N,N-dimethyl-3-(6-methyl-7-oxo-6,7-dihydro-1H-pyrrolo[2,3-c]pyridin-4-yl)benzamide | C17 H17 N3 O2 | 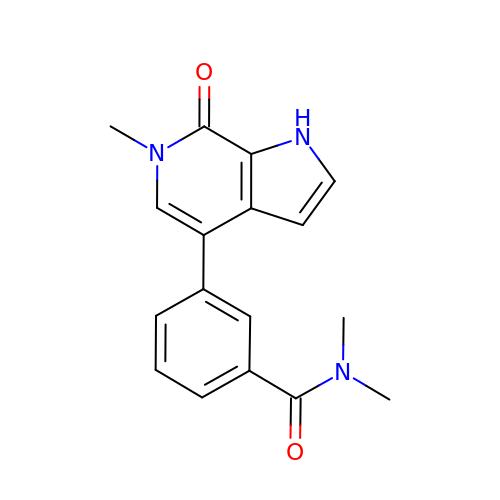YHMNROQTPUKNLA-UHFFFAOYSA-N> DGGSFWYR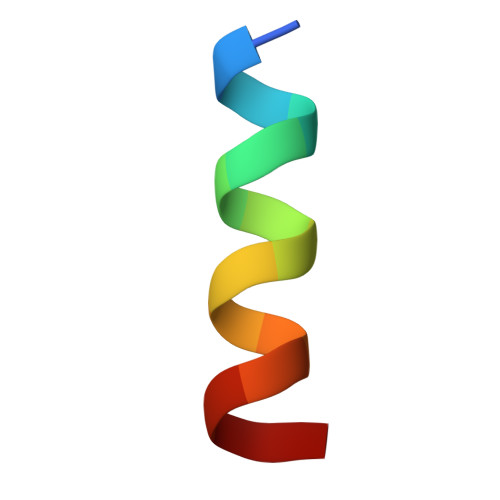AMKALYG We recently discovered that M-Sec, a 73-kDa cytosolic protein also known as tumor necrosis factor alpha-induced protein 2 (TNFaip2) or B949, plays a central role in inducing membrane protrusions during TNT formation. M-Sec-induced TNT formation is accompanied by actin cytoskeleton remodeling, which requires the association with RalA, a small GTPase, and its downstream effector, the exocyst complex10. We found that M-Sec binds phosphoinositides on the plasma membrane via its N-terminal polybasic region. We identified a conserved, positively charged surface in the C-terminal half that is essential for M-Sec interaction with active RalA and promotion of TNT formation by extending out the plasma membrane.

To obtain high resolution M-Sec structural information that might provide insight into the mechanism of membrane protrusion formation, we determined the crystal structure of the N-terminally truncated (residues 1–66) M-Sec at 3.0 Å resolution. Although we could also crystallize the full-length M-Sec, the N-terminal 66 residues are disordered and the corresponding electron density could not be observed. The structure consists entirely of α-helices and intervening loops of variable length, organized into a series of helix-bundle domains. This domain structure is similar to that of subunits of multi-subunit membrane tethering complexes (Exo70, Exo8416, Sec618, and Sec1529 of the exocyst complex, Tip20 and Dsl1 of the Dsl1 complex2030, Cog4 of the COG complex21, and Vps53 and Vps54 of the GARP complex2223) and cargo-binding domains of myosin V-family proteins. Particularly, there is a remarkable resemblance between the C-terminal halves of M-Sec and yeast Sec618 (Cα r.m.s.d of 3.0 Å over 278 amino acids), as expected from their high sequence similarity. The domain arrangement of M-Sec (domain A: Helix 1–4, domain B: Helix5–9, domain C: Helix9–13, domain D: Helix13–16) is similar to that of Exo70 and adopts a straight rod-like conformation. In addition, M-Sec has an extra C-terminal domain (domain E: Helix 17–20), which is conserved among tethering subunits and cargo-binding domains of myosin V 18202123303132. The calculated electrostatic surface potential of M-Sec revealed a positively charged surface that covers both domains D and E, where conserved lysine and arginine residues are widely distributed and exposed to solvent. To test this possibility, we introduced two sets of mutations that would decrease the overall positive charge in domains D and E: One set is a quadruple mutation K531A/R532A/R533A/K537A, and the other is a double mutation K470A/K474A. On the other hand, no binding of either M-Sec mutant to RalA was detected in the presence or absence of GTPγS or GDP, while the interaction of Sec8 with RalA in the presence of GTPγS was unaffected. These results suggest that the positively charged surface of domains D and E is responsible for the interaction with RalA, which is required for subsequent extension of the plasma membrane.

>GPLSDLEVQPKPRPELDGPLPTVEELKEALEHGRLEVAWQVLALERQLEAAAAAGGMSNEELVWRQSKVEALYVLLCDQVLGVLRRPLEAAPERLSQALAVVSQEELEDRRASGGPLAAALEATRPRRWLQRWRGVVAEVAAERLDAQPATAPEGRSEAESRFLHMGRTMKEDLEVVVERLKPLFPDEFNVVRTYAESYHYHFASHLCALAQFELCERDTYLLLLWVQNLYPNDILNSPKLAQELQGVGLGSLLPPKQIRLLEAMFLSNEVTSVKQLMARALELESQRWTQDVAPQSLDGHCHSELAIDILQIISQGQTKAENITSDVGMQIKQLLLVELAALLRSYQRAFDEFLEKSKLLRNYRVNIMANINNCLFFWTSVEQKWQISHDSLNRLLEPLKDLKAHGFDTLLQSLFLDLKPLFKKFTQTRWANPVETLEEIITTVSSSLPEFSELQDCFREELMETVHLHLVKEYIIRLCKRRLVLKTAEQQQQLARHILANADAIQGFCTENGSTATWLHRALPMIAEIIRLQDSSAIKIEVATYATWYPDFSKGHLNAILAIKGNLPSSEVRSIRNILDINTGVQEPPRPLFSLIKVT[2x]> MPFVNKQFNYKDPVNGVDIAYIKIPNAGQMQPVKAFKIHNKIWVIPERDTFTNPEEGDLNPPPEAKQVPVS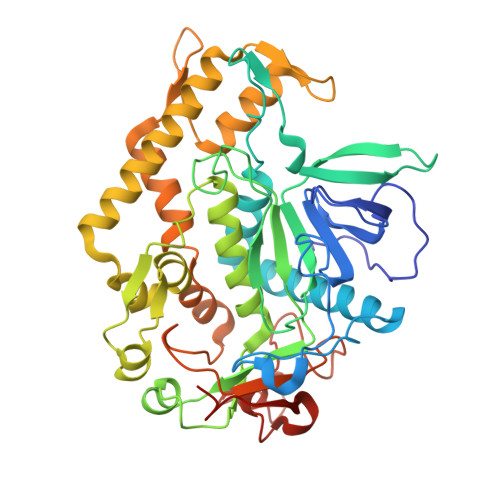YYDSTYLSTDNEKDNYLKGVTKLFERIYSTDLGRMLLTSIVRGIPFWGGSTIDTELKVIDTNCINVIQPDGSYRSEELNLVIIGPSADIIQFECKSFGHEVLNLTRNGYGSTQYIRFSPDFTFGFEESLEVDTNPLLGAGKFATDPAVTLAHELIHAGHRLYGIAINPNRVFKVNTNAYYEMSGLEVSFEELRTFGGHDAKFIDSLQENEFRLYYYNKFKDIASTLNKAKSIVGTTASLQYMKNVFKEKYLLSEDTSGKFSVDKLKFDKLYKMLTEIYTEDNFVKFFKVLNRKTYLNFDKAVFKINIVPKVNYTIYDGFNLRNTNLAANFNGQNTEINNMNFTKLKNFTGLFEHHHHHH>MDRRRFIKGSMAMAAVCGTSGIASLFSQAAFAADSDIADGQTQRFDFSILQSMAHDLAQTAWRGAPRPLPDTLATMTPQAYNSIQYDAEKSLWHNVENRQLDAQFFHMGMGFRRRVRMFSVDPATHLAREIHFRPELFKYNDAGVDTKQLEGQSDLGFAGFRVFKAPELARRDVVSFLGASYFRAVDDTYQYGLSARGLAIDTYTDSKEEFPDFTAFWFDTVKPGATTFTVYALLDSASITGAYKFTIHCEKSQVIMDVENHLYARKDIKQLGIAPMTSMFSCGTNERRMCDTIHPQIHDSDRLSMWRGNGEWICRPLNNPQKLQFNAYTDNNPKGFGLLQLDRDFSHYQDIMGWYNKRPSLWVEPRNKWGKGTIGLMEIPTTGETLNNIVCFWQPEKAVKAGDEFAFQYRLYWSAQPPVHCPLARVMATRTGMGGFSEGWAPGEHYPEKWARRFAVDFVGGDLKAAAPKGIEPVITLSSGEAKQIEILYIEPIDGYRIQFDWYPTSDSTDPVDMRMYLRCQGDAISETWLYQYFPPAPDKRQYVDDRVMSLEHHHHHH[12x]

Most Gram-negative bacteria synthesize osmo-regulated periplasmic glucans (OPG) in the periplasm or extracellular space. In this study, structural and functional analyses of OpgG and OpgD from Escherichia coli revealed that these proteins are β-1,2-glucanases with remarkably different activity from each other, establishing a new glycoside hydrolase family, GH186. Furthermore, a reaction mechanism with an unprecedentedly long proton transfer pathway among glycoside hydrolase families is proposed for OpgD. The conformation of the region that forms the reaction pathway differs noticeably between OpgG and OpgD, which explains the observed low activity of OpgG.

The ligand-free structure of EcOpgD was determined at 2.95 Å resolution. The overall structure of the ligand-free EcOpgD resembles that of the ligand-free EcOpgG. The substrate binding site is formed as a cleft in the ligand-free structure, whereas this site forms a tunnel in the structure of the complex. The difference arises mainly from the closure motion of α-helix 3 to the substrate in the cleft.> XETLTGQYDKNLVTTVE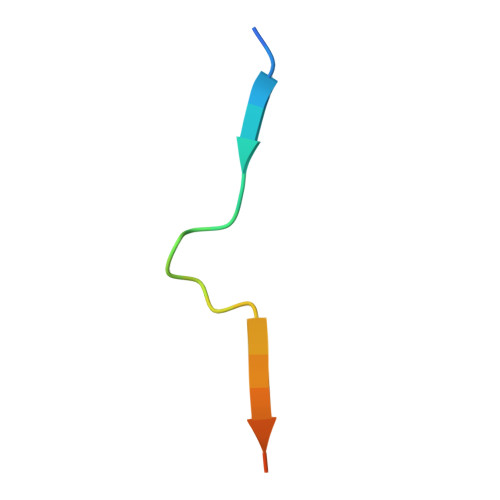EEYDSX>MQATVHESKQSIMQRILTVFVFTLLIATVGLFIGQFVPVALMLPLSILEVAMIILAFWMRRRKAVGYAFVYTFAFVSGITLFPIVSHYASIAGAYVVLEAFGSTFVIFAVLGTIGAKMKKDLSFLWSFLLVAVLALAVVGIFNIFSPLNSAAMMAYSVIGTIVFSLYILYELNQIKHRHITEDLIPVMALSLYLDFIN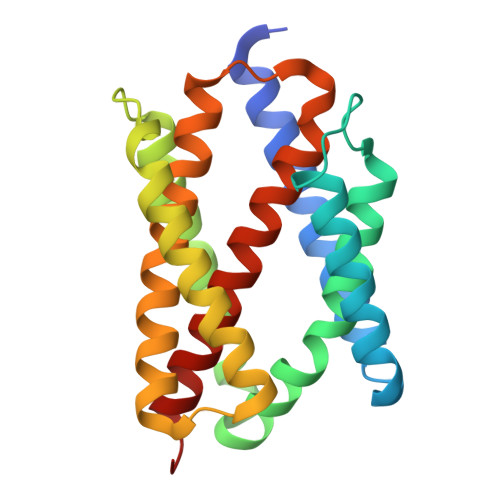LFINLLRFFGILSSDD[4x]>[3x]MPLLSASIVSAPVVTSETYVDIPGLYLDVAKAGIRDGKLQVILNVPTPYATGNNFPGIYFAIATNQGV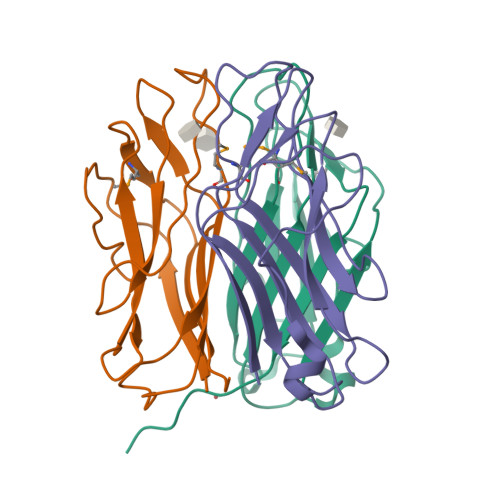VADGCFTYSSKVPESTGRMPFTLVATIDVGSGVTFVKGQWKSVRGSAMHIDSYASLSAIWGTAAPSSQGSGNQGAETGGTGAGNIGGG>[2x]QTLTLSPNLIGFNSNEGE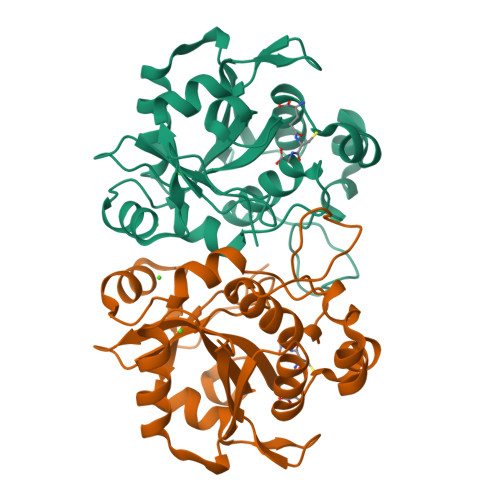KLLLTSRSREDFFPLSMQFVTQVNQAYSGVASIIMVLNSLGINAPETAQYSPYRVFTQDNFFSNEKTKAVIAPEVVARQGMTLDELGRLIASYGVKVKVNHASDTNIEDFRKQVAENLKQDGNFVIVNYLRKEIGQERGGHISPLAAYNEQTDRFLIMDVSRYKYPPVWVKTTDLWKAMNTVDSVSQKTRGFVFVSKTQD>[2x]LATTSDHDFSYLSFAYDATDLELEGSYDYVIVGGGTSGCPLAATLSEKYKVLVLERGSLPTAYPNVLTADGFVYNLQQEDDGKTPVERFVSEDGIDNVRGRVLGGTSIINAGVYARANTSIYSASGVDWDMDLVNQTYEWVEDTIVYKPNSQSWQSVTKTAFLEAGVHPNHGFSLDHEEGTRITGSTFDNKGTRHAADELLNKGNSNNLRVGVHASVEKIIFSNAPGLTATGVIYRDSNGTPHQAFVRSKGEVIVSAGTIGTPQLLLLSGVGPESYLSSLNIPVVLSHPYVGQFLHDNPRNFINILPPNPIEPTIVTVLGISNDFYQCSFSSLPFTTPPFGFFPSSSYPLPNSTFAHFASKVAGPLSYGSLTLKSSSNVRVSPNVKFNYYSNLTDLSHCVSGMKKIGELLSTDALKPYKVEDLPGVEGFNILGIPLPKDQTDDAAFETFCRESVASYWHYHGGCLVGKVLDGDFRVTGINALRVVDGSTFPYTP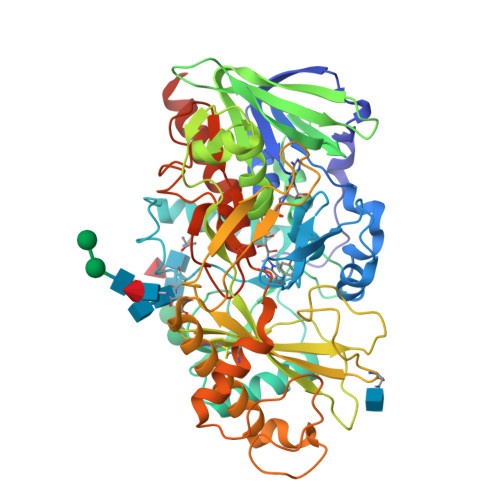ASHPQGFYLMLGRYVGIKILQERSASDLKILDSLKSAASLVL>MGHMNLTELKNTPVSELITLGENMGLENLARMRKQDIIFAILKQHAKSGEDIFGDGVLEILQDGFGFLRSADSSYLAGPDDIYVSPSQIRRFNLRTGDTISGKIRPPKEGERYFALLKVNEVNFDKPENARNKILFENLTPLHANSRLRMERGNGSTEDLTARVLDLASPIGRGQRGLIVAPPKAGKTMLLQNIAQSIAYNHPDCVLMVLLIDERPEEVTEMQRLVKGEVVASTFDEPASRHVQVAEMVIEKAKRLVEHKKDVIILLDSITRLARAYNTVVPASGKVLTGGVDANALHRPKRFFGAARNVEEGGSLTIIATALIDTGSKMDEVIYEEFKGTGNMELHLSRKIAEKRVFPAIDYNRSGTRKEELLTTQEELQKMWILRKIIHPMGEIDAMEFLINKLAMTKTNDDFFEM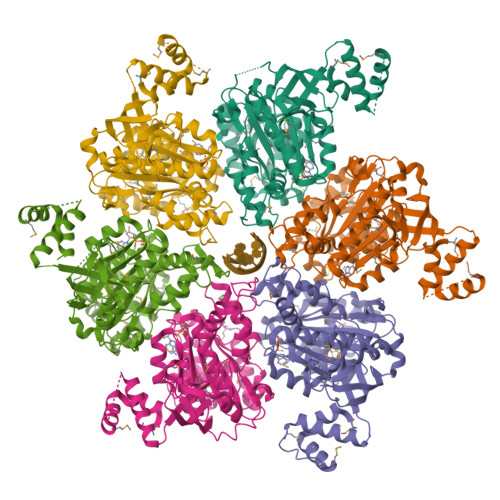MK[6x]>[2x]VKESSFVEKMKKTGRNIIVFYGSQTGTAEEFANRLSKDAHRYGMRGMSADPEEYDLADLSSLPEIDKSLVVFCMATYGEGDPTDNAQDFYDWLQETDVDLTGVKFAVFGLGNKTYEHFNAMGKYVDQRLEQLGAQRIFELGLGDDDGNLEEDFITW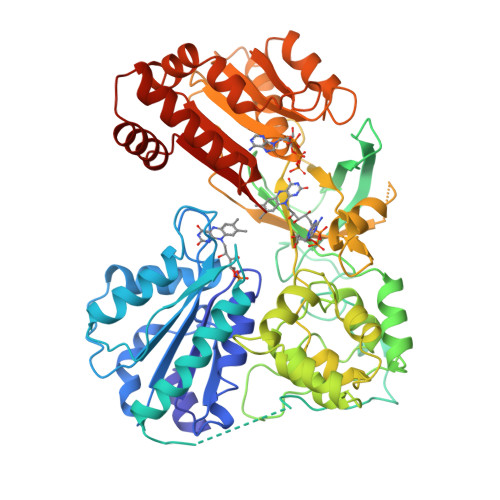REQFWPAVCEFFGVEATGEESSIRQYELVVHEDMDVAKVYTGEMGRLKSYENQKPPFDAKNPFLAAVTANRKLNQGTERHLMHLELDISDSKIRYESGDHVAVYPANDSALVNQIGEILGADLDVIMSLNNLDEESNKKHPFPCPTTYRTALTYYLDITNPPRTNVLYELAQYASEPSEQEHLHKMASSSGEGKELYLSWVVEARRHILAILQDYPSLRPPIDHLCELLPRLQARYYSIASSSKVHPNSVHICAVAVEYEAKSGRVNKGVATSWLRAKEPAGENGGRALVPMFVRKSQFRLPFKSTTPVIMVGPGTGIAPFMGFIQERAWLREQGKEVGETLLYYGCRRSDEDYLYREELARFHKDGALTQLNVAFSREQAHKVYVQHLLKRDREHLWKLIHEGGAHIYVCGDARNMAKDVQNTFYDIVAEFGPMEHTQAVDYVKKLMTKGRYSLDVWS>[2x]MHHHHHHHHENLYFQGGSST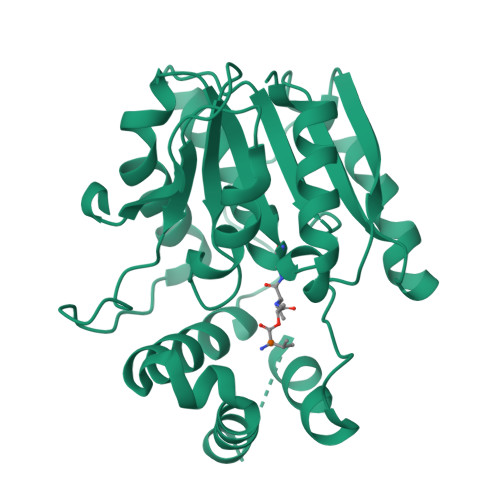AGDPTAKLVRLNPRGGDGPGIVFAPPAGGTVLGYIELARHLKGFGEIHGVEAPGLGAGETPVYPSFEEMVQFCSDSAAGVAGDGVYIGGHALGGHIAFYLATMLLDRGIRPKGLIILDTPPRLGDIPVADADLTEEETKVFILAMGIGGMLDQDRDALKDLPYEEAKQLLLDRAKNDPRVSAFLSEDYLDRFLRLQMHQLMYSRDVVLPQRKLDIPIHVFRTKNHAPEVARLFSAWENYAAGEVTFVDIPGDHATMLRAPHVSEVAQLLDRHCGLPSDDGPRG>MNNSNLAAA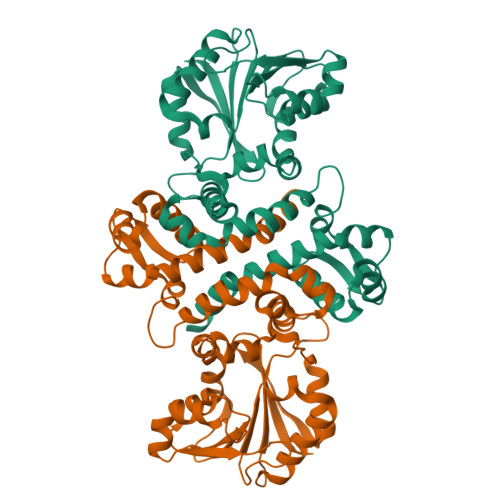RNLIQVVTGEWKSRCVYVATRLGLADLIESGIDSDETLAAAVGSDAERIHRLMRLLVAFEIFQGDTRDGYANTPTSHLLRDVEGSFRDMVLFYGEEFHAAWTPACEALLSGTPGFELAFGEDFYSYLKRCPDAGRRFLLAMKASNLAFHEIPRLLDFRGRSFVDVGGGSGELTKAILQAEPSARGVMLDREGSLGVARDNLSSLLAGERVSLVGGDMLQEVPSNGDIYLLSRIIGDLDEAASLRLLGNCREAMAGDGRVVVIERTISASEPSPMSVLWDVHLFMACAGRHRTTEEVVDLLGRGGFAVERIVDLPMETRMIVAARA[2x]Here we introduce RFpeptides, a denoising diffusion-based pipeline for designing macrocyclic binders against protein targets of interest. We tested 20 or fewer designed macrocycles against each of four diverse proteins and obtained binders with medium to high affinity against all targets. X-ray structures for macrocycle-bound myeloid cell leukemia 1, γ-aminobutyric acid type A receptor-associated protein and RbtA complexes match closely with the computational models, with a Cα root-mean-square deviation < 1.5 Å to the design models. RFpeptides is not limited to generating macrocycles with particular motifs or topologies; the diffusion process generates macrocycles with diverse shapes and sizes and selects the topologies appropriate for the protein being targeted. Among the four targets tested here, binders for MCL1 and MDM2 have helical motifs, binders for GABARAP have a β-sheet topology and binders for RbtA sample looplike conformations that make extensive contacts with the flat surface of this target.

We designed macrocycles against Rhombotarget A (RbtA), a recently identified cell surface protein from the ESKAPE pathogen, Acinetobacter baumannii. There are no experimentally determined structures available for this protein and sequence-based searches against the Protein Data Bank (PDB) did not return notable matches to other protein structures. We predicted the structure of the 617-aa full-length protein using AF2 and RF2; both methods predicted similar overall structures (Cα r.m.s.d. of 0.4 Å over 509 residues excluding the signal peptide and transmembrane domain) with high confidence (predicted local distance difference test (pLDDT) > 90). AF2 and RF2 both predicted two distinct extracellular domains: an N-terminal β-helix domain and a C-terminal Ig-like domain. We expressed the Avi-tagged version of the RbtA N-terminal domain (residues 20–458) and used it for binding screens using SPR. To confirm the structures of RbtA and RBB_D10 and the binding mode between them, we determined the high-resolution X-ray crystal structure of apo and macrocycle-bound RbtA using X-ray crystallography at 2 Å and 2.6 Å resolution, respectively. The apo structure of the RbtA N-terminal domain, which is also the first experimentally determined structure from this class of bacterial proteins, matched our AF2 and RF2 predictions for this target very closely, with an overall Cɑ r.m.s.d. of 1.2 Å and 1.1 Å between the X-ray structure of the RbtA N-terminal domain and the AF2-predicted and RF2-predicted structures, respectively.

>[2x]MGADIEVTTTIDEDVDNTVCSLREAVELINKRNSSDSTVVASVKDGYHGCGNKDASSNIILQRDKEYTLNSRITITAPLTISTAKNDSTLVDTDQPGSHNATIKMAGTDQLFKIDDESVEKASFSVLLSDLNLQGAGANSKVLTGGLILNHEKLTIQNSRLTGGYANQGGVIYNQGFASKSDRTFGFVYIVNSLIQNNKAAQGGVIYSEQPLFLITQSVIRDNEVSNTSGSLFFSQDSFDDESTGEYVVQRAIGLSNSTVFHNKGGFITNVRDGMFVNNITMIKNDKGLFLEAPQGNASISNSILVGNTINCQANSTDKAIIQSNLVTTECNRNASVKVPNILYPANQKLIAGSTDEGVCDVASKDGLLCPFNTPKDSFLGFFKPRLLESYNTLADSLIINKGRLYSDGTSVGLASCETLDQRGKRRTGYDELCDLGAIEYIGLNDIFEAQKIEWHELEHHHHHH> SSRTRRE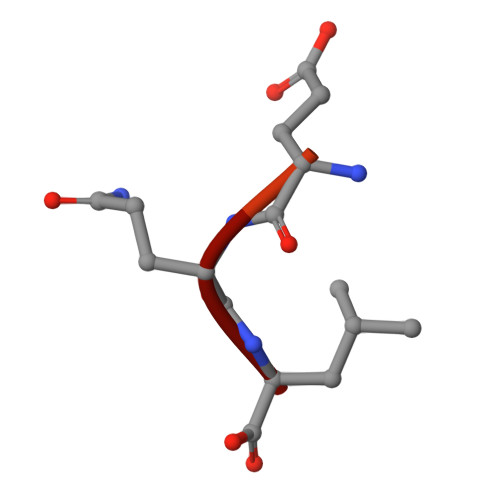EQL>SNAQFGGLPVPLDQTLPLNVNPALPLSPTGLAGSLTNALSNGLLSGGLLGILENLPLLDILKPGGGTSGGLLGGLLGKVTSVIPGLNNVIDIKVTDPQLLELGLVQSPDGHRLYVTIPLGIKLQVNTPLVGASLLRLAVKLDITAEIL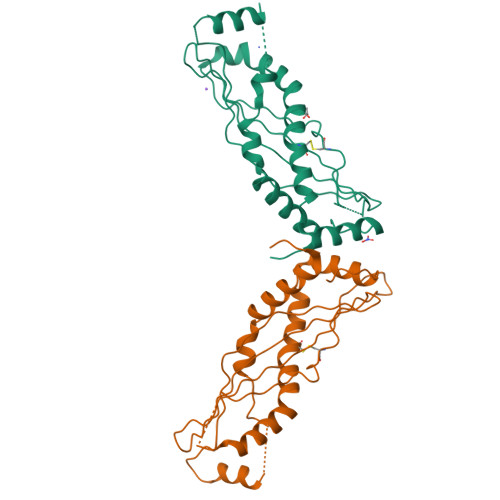AVRDKQERIHLVLGDCTHSPGSLQISLLDGLGPLPIQGLLDSLTGILNKVLPELVQGNVCPLVNEVLRGLDITLVHDIVNMLIHGLQFVIKV[2x]>SHVEYSRITKFFQEQPLEGYTLFSHRSAPNGFKVAIVLSELGFHYNTIFLDFNLGEHRAPEFVSVNPNARVPALIDHGMDNLSIWESGAILLHLVNKYYKETGNPLLWSDDLADQSQINAWLFFQTSGHAPMIGQALHFRYFHSQKIASAVERYTDEVRRVYGVVEMALAERREALVMELDTENAAAYSAGTTPMSQSRFFDYPVWLVGDKLTIADLAFVPWNNVVDRIGINIKIEFPEVYKWTKHMMRRPAVIKALRGE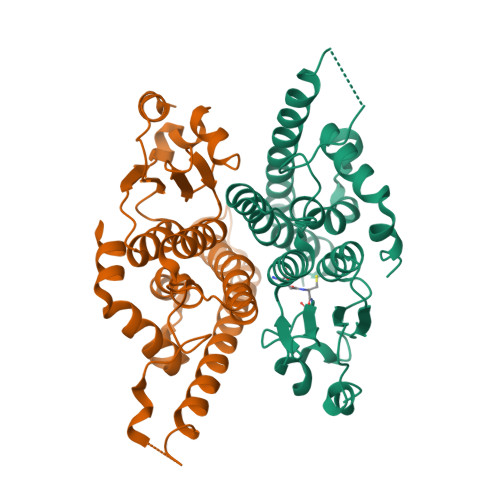[4x]> MGNNIEVIKMVEVKLENLTKRFGNFTAVNKLNLTIKDGEFLVLLGPSGCGKTTTLRMIAGLEEPTEGRIYFGDRDVTYLPPKDRNISMVFQSYAVWPHMTVYENIAFPLKIKKFPKDEIDKRVRWAAELLQIEELLNRYPAQLSGGQ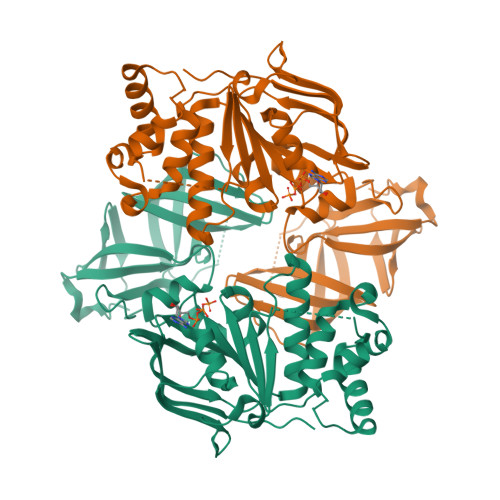RQRVAVARAIVVEPDVLLMDEPLSNLDAKLRVAMRAEIKKLQQKLKVTTIYVTHDQVEAMTMGDRIAVMNRGQLLQIGSPTEVYLRPNSVFVATFIGAPEMNILEVSVGDGYLEGRGFRIELPQDLMDLLKDYVGKTVLFGIRPEHMTVEGVSELAHMKRTARLIGKVDFVEALGTDTILHVKFGDELVKVKLPGHIPIEPGREVKVIMDLDMIHVFDKDTEKAIV>SLEPVKNIIHNSIDDLIDEFNLLENVSDELYELKKLNNLDEKYLISFEDISKNNSTYSVRFINKSNGESVYVETEKEIFSKYSEHITKEISTIKNSIITDVNGNLLDNIQLDHTSQVNTLNAAFFIQSLIDYSSNKDVLNDLSTSVKVQLYAQLFSTGLNTIYDSIQLVNLISNAVNDTINVLPTITEGIPIVSTILDGINLGAAIKELLDEHDPLLKKELEAKVGVLAINMSLSIAATVASIVGIGAEVTIFLLPIAGISAGIPSLVNNELILHDKATSVVNYFNHLSESKKYGPLKTEDDKILVPIDDLVISEIDFNNNSIKLGTCNILAMEGGSGHTVTGNIDHFFSSPSISSHIPSLSIYSAIGIETENLDFSKKIMMLPNAPSRVFWWETGAVPGLRSLENDGTRLLDSIRDLYPGKFYWRFYAFFDYAITTLKPVYEDTNIKIKLDKDTRNFIMPTITTNEIRNKLSYSFDGAGGTYSLLLSSYPISTNINLSKDDLWIFNIDNEVREISIENGTIKKGKLIKDVLSKIDINKNKLIIGNQTIDFSGDIDNKDRYIFLTCELDDKISLIIEINLVAKSYSLLLSGDKNYLISNLSNTIEKINTLGLDSKNIAYNYTDESNNKYFGAISKTSQKSIIHYKKDSKNILEFYNDSTLEFNSKDFIAEDINVFMKDDINTITGKYYVDNNTDKSIDFSISLVSKNQVKVNGLYLNESVYSSYLDFVKNSDGHHNTSNFMNLFLDNISFWKLFGFENINFVIDKYFTLVGKTNLGYVEFICDNNKNIDIYFGEWKTSSSKSTIFSGNGRNVVVEPIYNPDTGEDISTSLDFSYEPLYGIDRYINKVLIAPDLYTSLININTNYYSNEYYPEIIVLNPNTFHKKVNINLDSSSFEYKWSTEGSDFILVRYLEESNKKILQKIRIKGILSNTQSFNKMSIDFKDIKKLSLGYIMSNFKSFNSENELDRDHLGFKIIDNKTYYYDEDSKLVKGLININNSLFYFDPIEFNLVTGWQTINGKKYYFDINTGAALTSYKIINGKHFYFNNDGVMQLGVFKGPDGFEYFAPANTQNNNIEGQAIVYQSKFLTLNGKKYYFDNNSKAVTGWRIINNEKYYFNPNNAIAAVGLQVIDNNKYYFNPDTAIISKGWQTVNGSRYYFDTDTAIAFNGYKTIDGKHFYFDSDCVVKIGVFSTSNGFEYFAPANTYNNNIEGQAIVYQSKFLTLNGKKYYFDNNSKAVTGLQTIDSKKYYFNTNTAEAATGWQTIDGKKYYFNTNTAEAATGWQTIDGKKYYFNTNTAIASTGYTIINGKHFYFNTDGIMQIGVFKGPNGFEYFAPANTDANNIEGQAILYQNEFLTLNGKKYYFGSDSKAVTGWRIINNKKYYFNPNNAIAAIHLCTINNDKYYFSYDGILQNGYITIERNNFYFDANNESKMVTGVFKGPNGFEYFAPANTHNNNIEGQAIVYQNKFLTLNGKKYYFDNDSKAVTGWQTIDGKKYYFNLNTAEAATGWQTIDGKKYYFNLNTAEAATGWQTIDGKKYYFNTNTFIASTGYTSINGKHFYFNTDGIMQIGVFKGPNGFEYFAPANTDANNIEGQAILYQNKFLTLNGKKYYFGSDSKAVTGLRTIDGKKYYFNTNTAVAVT[2x]

Two homologous exotoxins, toxin A (TcdA) and B (TcdB), are the key virulence factors of C. difficile, leading to C. difficile infections (CDI) with variable clinical features including life-threatening pseudomembranous colitis. Most of these toxins are composed of four structural modules: an N-terminal glucosyltransferase domain (GTD), followed by a cysteine protease domain (CPD), a delivery and receptor-binding domain (DRBD), and a large C-terminal combined repetitive oligopeptides domain (CROPs). Triggered by acidification in the endosomes, the hydrophobic pore-forming region of the toxin undergoes membrane insertion and facilitates the translocation of the GTD and the CPD into the cytosol. The GTD then glucosylates and inactivates the Rho and/or Ras families of small guanosine triphosphatases (GTPases) in host cells, resulting in depolymerization of the actin cytoskeleton, cell rounding, and ultimately cell death.

Here, we report a 3.18-Å resolution crystal structure of a TcdA fragment composed of DRBD and CROPs I–V (residues L843-T2481, referred to as DRBD-5CROPs), which serves as the foundation for us to piece together all the known fragment structures of TcdA into a complete structure of TcdA holotoxin. The crystal structure of DRBD-5CROPs was solved by molecular replacement (see the Materials and Methods section), and a near complete structure including residues 855–2,481 was built except for a small flexible region including residues 1,661–1,667 that had no visible electron density. The structure of DRBD-5CROPs starts with an N-terminal small globular subdomain (SGS, residues 850–1,025) that is part of the DRBD but with a largely unknown function. Notably, a hydrophobic region buried in the SGS (residues 958–1,039) is considered to be the N-terminal portion of the pore-forming region (PFR, residues 958–1,130) on TcdA, and the rest of PFR then extends away from the SGS forming four α-helices (PFR-α1 to α4, residues 1,040–1,130) that stretch across the elongated DRBD. The N-terminus of the CROPs is connected via a hinge region (residues 1,789–1,831) to the proximal tip of the DRBD where the SGS is localized. The CROPs I to IV then forms an arch-like structure pointing to the distal tip of the DRBD, where the first and second SRs and LR4 of CROPs IV interact with the DRBD. The rest of the CROPs IV-V kinks by ∼35° and extends further away from the DRBD. We found that a well-defined β-hairpin in the SGS of DRBD-5CROPs (residues 937–953) directly interacts with PFR-α1 and α2. We envision that the β-hairpin in the SGS in the closed form of TcdA can help to stabilize PFR-α1 and α2 in the DRBD-shielded conformation at neutral pH. Interestingly, we found that three residues in PFR-α4 (D1117, K1118, and T1120) interact with H2234, T2247, and E2259 in the CROPs IV via van del Waals interactions, suggesting that the CROPs can help stabilize the pore-forming region at interface II in the closed conformation.>MAKPIADDIVVRQVDVGETEQLMTFLLAHYYPEEPLTAGTHPPEPEAADKEFLLSNVPFGTCFVALHEGRIVAAVVAGPKDSHEPEHMAEEARKYAGGKWGSILHLLSAVETATDVCRRFSVPSCLHVHALGVDPQLRGRNLGGRLMETVAQRGR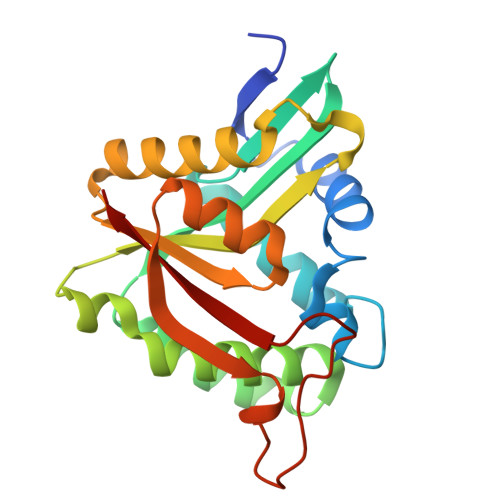DLGHQLVSVDCTSVYSARLVQRLGYQLINTLRYVDHLDASGQQVIRPPPPHESVQTFVLHL[2x]>MLPHGLIVSCQALPDEPLHSSFIMSKMALAAYEGGAVGIRANTKEDILAIKETVDLPVIGIVKRDYDHSDVFITATSKEVDELIESQCEVIALDATLQQRPKETLDELVSYIRTHAPNVEIMADIATVEEAKNAARLGFDYIGTTLHGYTSYTQGQLLYQNDFQFLKDVLQSVDAKVIAEGNVITPDMYKRVMDLGVHCSVVGGAITRPKEITKRFVQIMED[2x]

The third step in the sialic acid catabolic pathway is mediated by the enzyme N-acetylmannosamine-6-phosphate 2-epimerase (NanE), which catalyzes an inversion of stereochemistry at the C2 position of N-acetylmannosamine-6-phosphate (ManNAc-6P), yielding N-acetylglucosamine-6-phosphate (GlcNAc-6P). The crystal structure of NanE from Staphylococcus aureus, which comprises a triosephosphate isomerase barrel fold with an unusual dimeric architecture, was solved with both natural and modified substrates. NanE is essential for the growth of S. aureus in media containing N-acetylneuraminic acid as the sole carbon source and has a highly conserved active site across both Gram-positive and Gram-negative bacteria. Based on our structural and kinetic data, we propose that NanE performs its epimerization reaction using a novel proton displacement mechanism mediated by the substrate.

We aimed to examine the involvement of the C5 hydroxyl of ManNAc-6P in the catalytic mechanism. Two derivatives were synthesized with substitutions at the C5 hydroxyl: 5-deoxy-ManNAc-6P, with a substituted hydrogen, and 5-methyl-ManNAc-6P, with a substituted methoxy group. SaNanE was cocrystallized with these ligands to obtain ligand-bound structures. Unambiguous density for the N-acetyl and phosphate groups of the ligand was present in one of the monomers in the same position as in ManNAc-6P. The ligand was fit to an occupancy of 0.66 with phenix.refine, with citrate fitted to an occupancy of 0.34. The center of the ligand appears to bind in a different orientation to that of ManNAc-6P, notably with Glu180 interacting with the C4 hydroxyl of the substituted ligand. With the ability to form a hydrogen bond at the C5 position removed in 5-deoxy-ManNAc-6P, Glu180 has formed a short hydrogen bond (2.5 Å) with a different hydroxyl group. Mutagenesis studies identified the roles of Lys63 and Glu180, and crystallographic modeling highlighted the unusually short hydrogen bond between Glu180 and the substrate, which is retained even if the C5 hydroxyl of the substrate is removed (it now forms with the C4 hydroxyl).> SGIVQQQNNLLRAIEAQQHLLQLTVWGIKQLQARSGGRGGWMEWDREINNYTSLIHS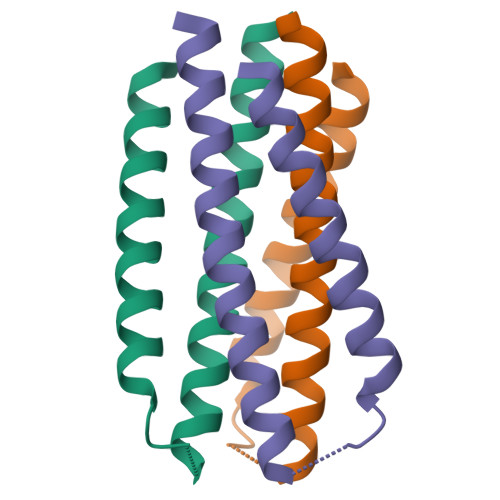LIEESQNLQEK RIFIN, a large family of Plasmodium variant surface antigens, plays a crucial role in malaria pathogenesis by mediating immune suppression through activation of inhibitory receptors such as LAIR1, and antibodies with LAIR1 inserts have been identified that bind infected erythrocytes through RIFIN. RIFIN also mediates immune suppression through activation of inhibitory immune receptors including leukocyte-associated immunoglobulin-like receptor 1 (LAIR1) and leukocyte immunoglobulin-like receptor B1 (LILRB1). Notably, human monoclonal antibodies that contain LAIR1-domain insertions in either switch region or between V and DJ regions have been isolated from donors, who have had malaria. To define the structural basis underpinning interactions between wild-type and antibody-inserted LAIR1 and polymorphic RIFIN, we investigated the overall architecture of three types of LAIR1-inserted antibodies, determined crystal structures of LAIR1 in complex with the RIFIN-interactive regions from two RIFINs (PF3D7_1040300 and PF3D7_0401300), and used the resultant structural information to derive a LAIR1-binding signature and to identify RIFINS from diverse Plasmodium species capable of recognizing LAIR1.

Phylogenetic analysis of the RIFIN-V2 apex sequence revealed two additional 3D7 RIFINs, referred to as RIF3 (PF3D7_0401300) and RIF4 (PF3D7_0401200), to be in the same branch as the initially identified LAIR1-positive RIFINs (RIF1 and RIF2). A similar approach also identified seven RIFINs in non-3D7 strains. Co-immunoprecipitation (co-IP) assays confirmed LAIR1 interaction with the newly identified 3D7 RIFINs, RIF3 and RIF4, and with three of the non-3D7 RIFINs. To provide insight into the recognition of these RIFINs, we determined the structure of the RIF3-V2 domain in complex with MGD21 LAIR1 at 2.5 Å resolution. The RIF3-LAIR1 structure resembled that of RIF1-LAIR1 with an overall rmsd of 1.46 Å over 546 Cα atoms, despite clear diversity in the primary RIFIN sequences at the binding interface. Structural analysis and sequence comparison of the LAIR1-RIFIN complex suggested a set of four conserved residues contributing to LAIR1-binding capacity, including residues D247, C254, C265 and R268. The interface between RIFIN-V2 apex and LAIR1 C-C’ region largely comprises hydrophobic interactions and backbone-mediated hydrogen bonds, and the interface is facilitated by an induced conformational fit of flexible RIFIN-V2 apex loops.

>[2x]TDLPRPSISAEPGTVIPLGSHVTFVCRGPVGVQTFRLERERNYLYSDTEDVSQTSPSESEARFRIDSVNAGNAGLFRCIYYKSRKWSEQSDYLELVVKGEDVTWA;>TDAIAAATKAAMIEGAAQGAVAGEAAGRNAIIGALKRYFHIDNLNGTSLKSFFNSTSYSDVTTIASAIDTQMTASCDAFSGKIVNQAFCDVRKTLRIVADPGKSFVKQKDAITGAVTQLVEKAKDTASFKATEVSSATSSKIITKQNALIE[2x]> SNASDKGKLSLQDVAELIRARACQRVVVMVGAGISTPSGIPDFRSPGSGLYSNLQQYDLPYPEAIFELPFFFHNPKPFFTLAKELYPGNYKPNVTHYFLRLLHDKGLLLRLYTQNIDGLERVSGIPASKLVEAHGTFASATCTVCQRPFPGEDIRADVMADRVPRCPVCTGVVKPDIVFFGEPLPQRFLLHVVDFPMADLLLILGTSLEVEPFASLTEA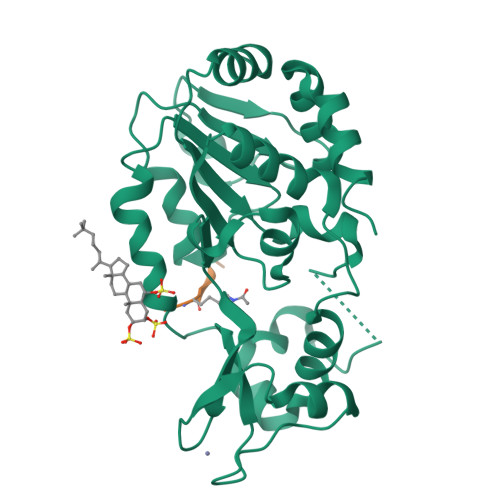VRSSVPRLLINRDLVGPLAWHPRSRDVAQLGDVVHGVESLVELLGWTEEMRDLVQRETGKLDGPDK;> TRSGKVMRRLRR> MEKTTEGAFYTREYRNLFKEFGYSEAEIQERVKDTWEQLFGDNPETKIYYEVGDDLGYLLDTGNLDVRTEGMSYGMMMAVQMDRKDIFDRIWNWTMKNMYMTEGVHAGYFAWSCQPDGTKNSWGPAPDGEEYFALALFFASHRWGDGDEQPFNYSEQARKLLHTCVHNGEGGPGHPMWNRDNKLIKFIPEVEFSDPSYHLPHFYELFSLWANEEDRVFWKEAAEASREYLKIACHPETGLAPEYAYYDGTPNDEKGYGHFFSGSYRVAANIGLDAEWFGGSEWSAEEINKIQAFFADKEPEDYRRYKIDGEPFEEKSLHPVGLIATNAMGSLASV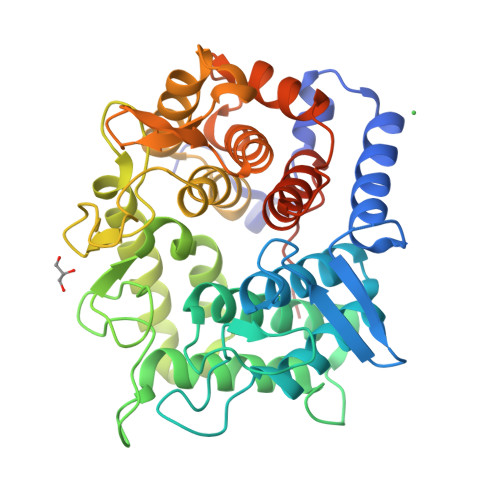DGPYAKANVDLFWNTPVRTGNRRYYDNCLYLFAMLALSGNFKIWFPEGQEEEHLEHHHHHH>GSHMAQDDPRYTKFLTQHYDAKPKGRDARYCESMMRRRGLTSPCKEVNTFIHGNKGSIKAICGANGSPYGENLRISQSPFQITTCKHTGGSPRPPCRYRASAGFRHV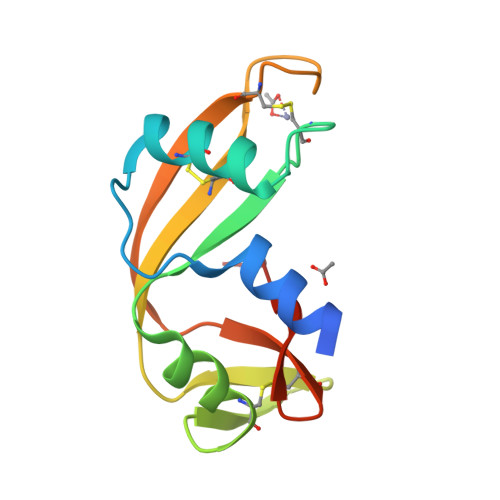VIACENGLPVHFDESFISL[2x]> MKILRTPDSRFANLPDYNFDPHYLMVDDSEDSELRVHYLDEGPRDADPVLLLHGEPSWCYLYRKMIPILTAAGHRVIAPDLPGFGRSDKPASRTD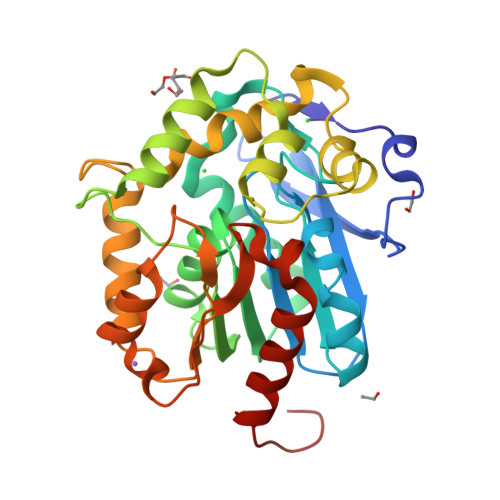YTYQRHVNWMQSVLDQLDLNNITLFCQDWGGLIGLRLVAENPDRFARVAAGNTMLPTGDHDLGEGFRKWQQFSQEIPQFHVGGTIKSGTVTKLSQAVIDAYNAPFPDESYKEGARQFPLLVPSTPDDPASENNRAAWIELSKWTKPFITLFSDSDPVTAGGDRIMQKIIPGTKGQAHTTIANGGHFLQEDQGEKVAKLLVQFIHDNPRHHHHHH>MSQTHKHAIPANIADRCLINPEQYETKYKQSINDPDTFWGEQGKILDWITPYQKVKNTSFAPGNVSIKWYEDGTLNLAANCLDRHLQENGDRTAIIWEGDDTSQSKHISYRELHRDVCRFANTLLDLGIKKGDVVAIYMPMVPEAAVAMLACARIGAVHSVIFGGFSPEAVAGRIIDSSSRLVITADEGVRAGRSIPLKKNVDDALKNPNVTSVEHVIVLKRTGSDIDWQEGRDLWWRDLIEKASPEHQPEAMNAEDPLFILYTSGSTGKPKGVLHTTGGYLVYAATTFKYVFDYHPGDIYWCTADVGWVTGHSYLLYGPLACGATTLMFEGVPNWPTPARMCQVVDKHQVNILYTAPTAIRALMAEGDKAIEGTDRSSLRILGSVGEPINPEAWEWYWKKIGKEKCPVVDTWWQTETGGFMITPLPGAIELKAGSATRPFFGVQPALVDNEGHPQEGATEGNLVITDSWPGQARTLFGDHERFEQTYFSTFKNMYFSGDGARRDEDGYYWITGRVDDVLNVSGHRLGTAEIESALVAHPKIAEAAVVGIPHAIKGQAIYAYVTLNHGEEPSPELYAEVRNWVAKEIGPLAT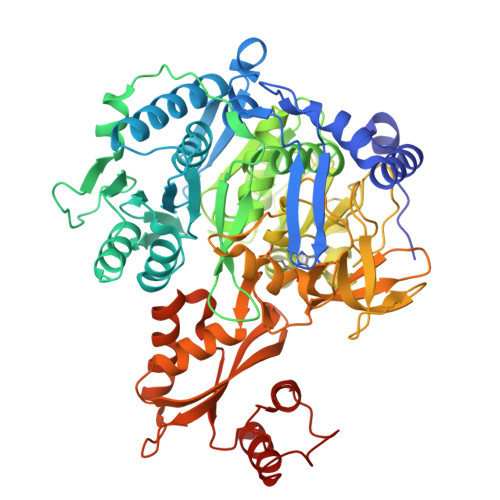PDVLHWTDSLPKTRSGKIMRRILRKIAAGDTSNLGDTSTLADPGVVEKLLEEKQAIAMPS[2x]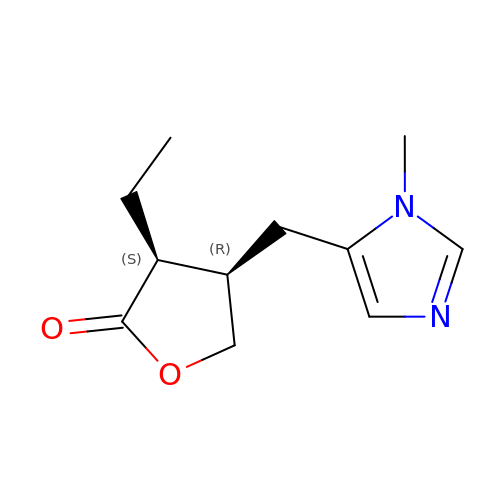(3S,4R)-3-ethyl-4-[(1-methyl-1H-imidazol-5-yl)methyl]dihydrofuran-2(3H)-one | C11 H16 N2 O2 | QCHFTSOMWOSFHM-WPRPVWTQSA-N Crenactins, restricted to Crenarchaea, are more closely related to actin than bacterial MreB. Actins’ primary function seems to be regulated polymerisation into cytomotive filaments and for this they contain an ATPase that is sensitive to the polymerisation state. The exact biological function of crenactins is currently unknown, however they were found to be located in functional clusters with other genes, including SMC proteins (Structural Maintenance of Chromosomes), highlighting possible roles in DNA dynamics, for example. Here we show the crystal structure of crenactin from Pyrobaculum calidifontis at 3.2 Å resolution.

The best conditions yielded crystals that belong to space group P41212 with a very long c-axis and diffract to 3.2 Å only, with the additional complication that diffraction is fairly anisotropic perpendicular to the long axis. Since each asymmetric unit in the two forms Natives 1 and 2 contained two monomers, it yielded 4-fold averaging, greatly improving the very poor phases coming from the weak molecular replacement solutions. This enabled automatic model building and manual rebuilding and refinement, using 2-fold non-crystallographic symmetry, to produce a high confidence structure, refined at 3.2 Å resolution with good R-factors and geometry. The structure of crenactin shows several loops that are longer than in actin, but overall, crenactin is closely related to eukaryotic actin, with an RMSD of 1.6 Å. Although crenactin is very closely related to eukaryotic actin in structure, crenactin’s sequence is longer than actin’s (432 for crenactin vs. 375 for yeast actin) and the extra residues are consumed to make a number of surface loops bigger. This is most pronounced in loops 295–322, which corresponds to a loop in actin that is involved in the formation of double helical filaments and has also been termed the ‘hydrophobic plug’. The crystals of crenactin have a very long c axis because they contain essentially infinite helical protofilaments. Eight subunits form a complete turn of 360° over a distance of 419 Å, the length of the unit cell of the crystals. This means that each subunit repeat is 52.4 Å and the angle from subunit to subunit is 45°. The helix is right-handed, as for actin filaments. The crenactin crystals contain a protofilament, made out of a single strand of crenactin subunits and this leads to an overall protofilament thickness of only 70 Å.

>[2x]MGVISDAYRLKYTFGVDFGTSYVKYGPITLNEPKMVQTRGLFLRDLPESVKMRIPPDVLARGLVVGDEEVRKYLSSVRDVQRNLKYPLKDGVARRDDEEAWRVLKELARYTLAQFPVSDPEFAGWLVAVALSALAPDYMYKAIFDIYDELASEFKIYAVTILPQPLAVAIAENAVNCVIVEGGHGNIQVAPISFALIREGLVALNRGGAEANAITREILKDIGYSDIAREEYAVEVVKRAVGLVPRRLKEAIRAAKSDPDRFVTKVRLSPVVEVEIPREYAWTRFLIGEIVFDPNHEEIKSYIEQSRLRIENAVIGDVTLYGEMDVASAIITSLRNVSVEIQERVASQIILSGGAFSWRVPPGMEDVAADSVTRVKIALEEKSPALASKVEVRLVSEPQYSVWRGAVIYGYALPLSLEWSDTTREGWRFPRR>AWITAPVALREGEDLSKKNPIAKIHSDLAEERGLKITYKYTGKGITEPPFGIFVFNKDTGELNVTSILDREETPFFLLTGYALDARGNNVEKPLELRIKVLDINDNEPVFTQDVFVGSVEELSAAHTLVMKINATDADEPNTLNSKISYRIVSLEPAYPPVFYLNKDTGEIYTTSVTLDREEHSSYTLTVEARDGNGEVTDKPVKQAQVQIRILDVNDNIPVVENKVLEGMVEENQVNVEVTRIKVFDADEIGSDNWLANFTFASGNEGGYFHIETDAQTNEGIVTLIKEVDYEEMKNLDFSVIVANKAAFHKSIRSKYKPTPIPIKVKVKNVKEGIHFKSSVISIYVSESMDRSSKGQIIGNFQAFDEDTGLPAHARYVKLEDRDNWISVDSVTSEIKLAKLPDFESRYVQ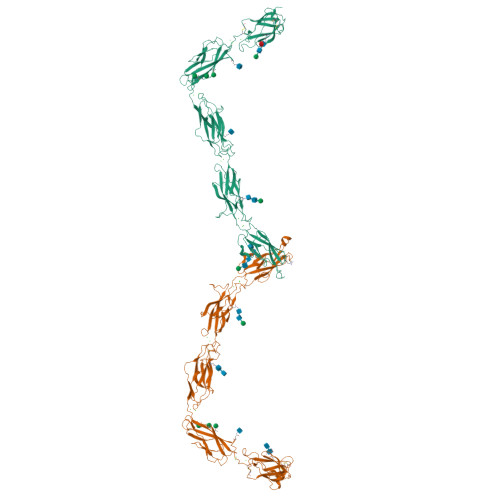NGTYTVKIVAISEDYPRKTITGTVLINVEDINDNCPTLIEPVQTICHDAEYVNVTAEDLDGHPNSGPFSFSVIDKPPGMAEKWKIARQESTSVLLQQSEKKLGRSEIQFLISDNQGFSCPEKQVLTLTVCECLHGSGCREAHHHHHH[2x]> GSHMASTPANVNSGPTSPVGGTRSAFS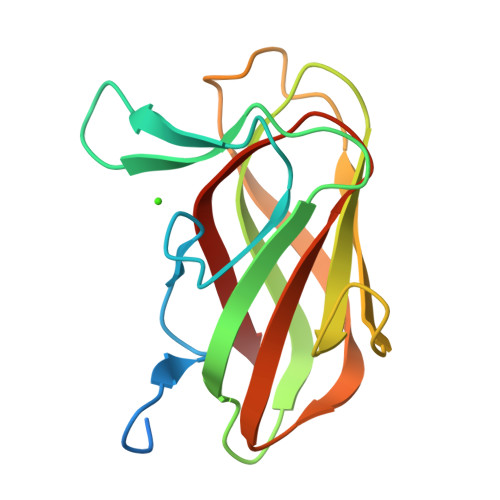NIQAEDYDSSYGPNLQIFSLPGGGSAIGYIENGYSTTYKNIDFGDGATSVTARVATQNATTIQVRLGSPSGTLLGTIYVGSTGSFDTYRDVSATISNTAGVKDIVLVFSGPVNVDWFVFSKSGT>AKPQIPKDKSKVAGYIEIPDADIKEPVYPGPATPE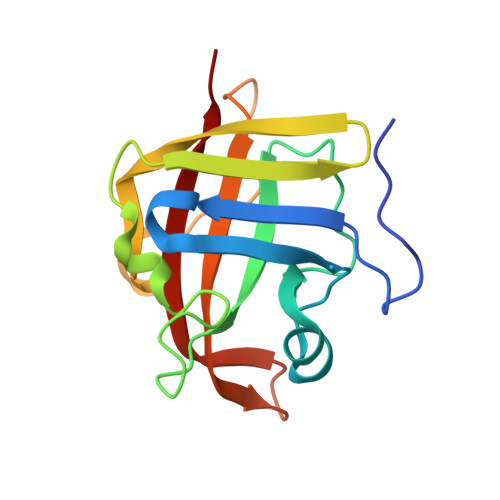QLNRGVSFAEENESLDDQNISIAGHTFIDRPNYQFTNLKAAKKGSMVYFKVGNETRKYKMTSIRDVKPTDVGVLDEQKGKDKQLTLITCDDYNEKTGVWEKRKIFVATEVK[3x]> DLKKNEDLKQMLESNKDSAKLDAMKRIVGMIAKGKNASELFPAVVKNVASKNIEIKKLVYVYLVRYAEEQQDLALLSISTFQRALKDPNQLIRASALRVLSSIRVPIIVPIMMLAIKEASADLSPYVRKNAAHAIQKLYSLDPEQKEMLIEVIEKLLKDKSTLVAGSVVMAFEEVCPDRIDLIHKNYRKLCNLLVDVEEWGQVVIIHMLTRYARTQFVSPWDPDHRLLIRNTKPLLQSRNAAVVMAVAQLYWHISPKSEAGIISKSLVRL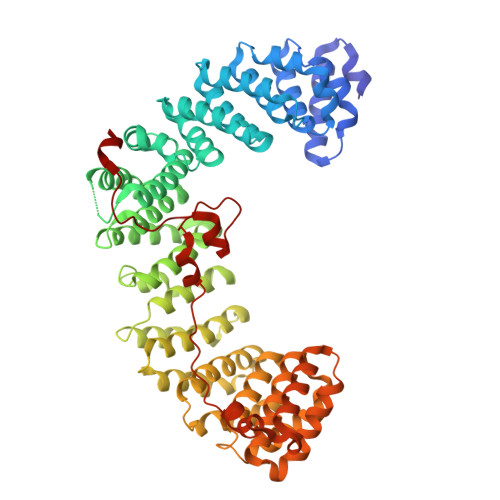LRSNREVQYIVLQNIATMSIQRKGMFEPYLKSFYVRSTDPTMIKTLKLEILTNLANEANISTLLREFQTYVKSQDKQFAAATIQTIGRCATNILEVTDTCLNGLVCLLSNRDEIVVAESVVVIKKLLQMQPAQHGEIIKHMAKLLDSITVPVARASILWLIGENCERVPKIAPDVLRKMAKSFTSEDDLVKLQILNLGAKLYLTNSKQTKLLTQYILNLGKYDQNYDIRDRTRFIRQLIVPNVKSGALSKYAKKIFLAQKPAPLLESPFKDRDHFQLGTLSHTLNIKATGYLELSNWPEVAPDPSVRN>[6x]MAHHH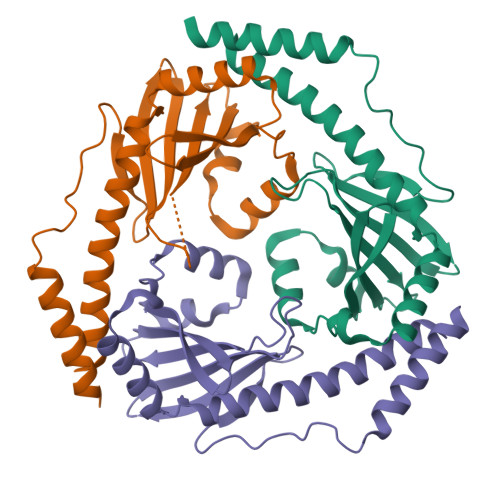HHHMSAPTALTVPRRSASDAALADATRRELEEEMGRSDKPEQPTPPAGWQVVRKPGTCTFDLTKSFEGEDLVVRYSTNQDSDKANSHNIFVYITQKNGQTMQADLSIEEGELVLNNIRFYDEAALAKDTGAEAEAKRNELYTGPLVHELDYDLLNCVMTYLEKRGVDEKLGEFVVLYSFWAEQQDYEAWLTTMNKFAS> RSPWDYKDDDDKLAAANSSIPESWEPCVEVVPNITYQCMELNFYKIPDNLPFSTKNLDLSFNPLRHLGSYSFFSFPELQVLDLSRCEIQTIEDGAYQSLSHLSTLILTGNPIQSLALGAFSGLSSLQKLVAVETNLASLENFPIGHLKTLKELNVAHNLIQSFKLPEYFSNLTNLEHLDLSSNKIQSIYCTDLRVLHQMPLLNLSLDLSLNPMNFIQPGAFKEIRLHKLTLRNNFDSLNVMKTCIQGLAGLEVHRLVLGEFRNEGNLEKFDKSALEGLCNLTIEEFRLAYLDYYLDGIIDLFNCLTNVSSFSLVSVTIERVKDFSYNFGWQHLELVNCKFGQFPTLKLKSLKRLTFTSNKGGNAFSEVDLPSLEFLDLSRNGLSFKGCC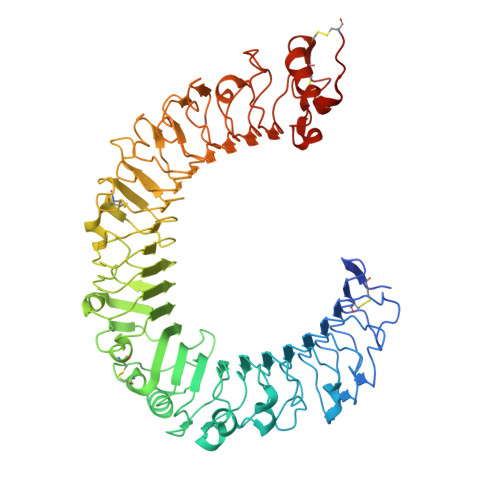SQSDFGTISLKYLDLSFNGVITMSSNFLGLEQLEHLDFQHSNLKQMSEFSVFLSLRNLIYLDISHTHTRVAFNGIFNGLSSLEVLKMAGNSFQENFLPDIFTELRNLTFLDLSQCQLEQLSPTAFNSLSSLQVLNMSHNNFFSLDTFPYKCLNSLQVLDYSLNHIMTSKKQELQHFPSSLAFLNLTQNDFACTCEHQSFLQWIKDQRQLLVEVERMECATPSDKQGMPVLSLNITCQMTGHHHHHH>AECSVDSQGNDQMQFNTNAITVDKSCKQFTVNLSHPGNLPKNVMGHNWVLSTAADMQGVVTDGMASGLDKDYLKPDDSRVIAHTKLIGSGEKDSVTFDV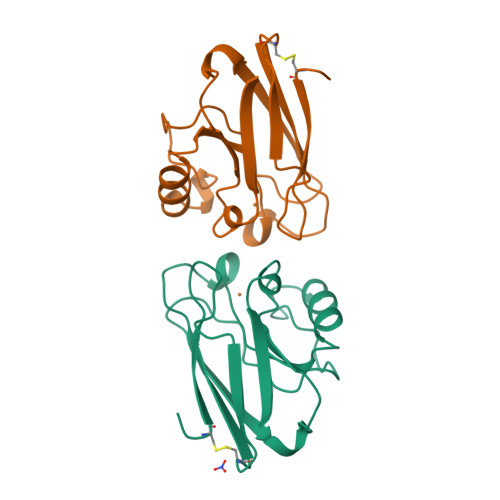SKLKEGEQYMFFCTFPGHSALMKGTLTLK[4x]> SYQSTCGLRQ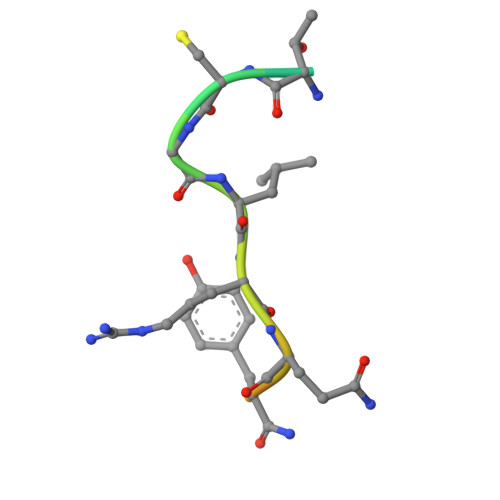YSQRQRR> MSDQEAKPSTEDLGDKKEGEYIKL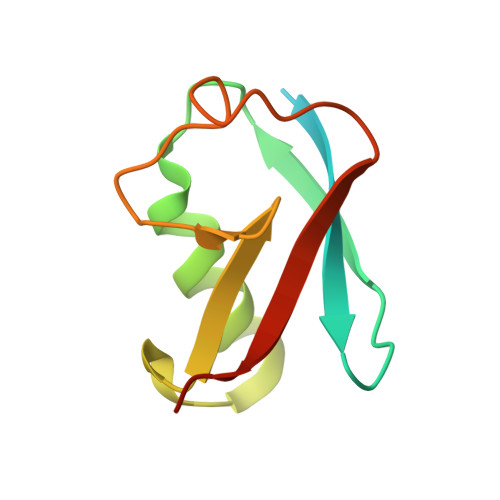KVIGQDSSEIHFKVKMTTHLKKLKESYCQRQGVPMNSLRFLFEGQRIADNHTPKELGMEEEDVIEVYQEQTGG> LPTQPRDIENFNSTQKFIEDNIEYITIIAFAQYVQEATFEEMEKLVKDMVEYKDRCMADKTLPECSKLPNNVLQEKICAMEGLPQKHNFSHCCSKVDAQRRLCFFYNKKSDVGFLPPFPTLDPEEKCQAYESNRESLLNHFLYEVARRNPFVFAPTLLTVAVHFEEVAKSCCEEQNKVNCLQTRAIPVTQYLKAFSSYQKHVCGALLKFGTKVVHFIYIAILSQKFPKIEFKELISLVEDVSSNYDGCCEGDVVQCIRDTSKVMNHICSKQDSISSKIKECCEKKIPERGQCIINSNKDDRPKDLSLREGKFTDSENVCQERDADPDTFFAKFTFEYSRRHPDLSIPELLRIVQIYKDLLRNCCNTENPPGCYRYAEDKFNETTEKSLKMVQQECKHFQNLGKDGLKYHYLIRLTKIAPQLSTEELVSLGEKMVTAFTTCCTLSEEFAC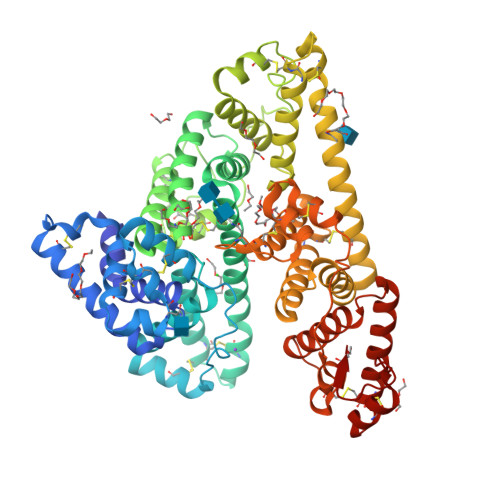VDNLADLVFGELCGVNENRTINPAVDHCCKTNFAFRRPCFESLKADKTYVPPPFSQDLFTFHADMCQSQNEELQRKTDRFLVNLVKLKHELTDEELQSLFTNFANVVDKCCKAESPEVCFNEESPKIGNKGENLYFQ> GPHMASMLEAKFEEASLFKRIIDGFKDCVQLVNFQCKEDGIIAQAVDDSRVLLVSLEIGVEAFQEYRCDHPVTLGMDLTSLSKILRCGNNTDTLTLIADNTPDSIILLFEDTKKDRIAEYSLKLMDIDADFLKIEELQYDSTLSLPSSEFSKIVRDLSQLSDSINIMITKETIKFVADGDIGSGSVIIKPFVDMEHPETSIKLEMDQPVDLTFGAKYLLDIIKGSSLSDRVGIRLSSEAPALFQFDLKSGFLQFFLAPKFNDEGSNSQSNGSGALEAKFEEASLFKRIIDGFKDCVQLVNFQCKEDGIIAQAVDDSRVLLVSLEIGVEAFQEYRCDHPVTLGMDLTSLSKILRCGNNTDTLTLIADNTPDSIILLFEDTKKDRIAEYSLKLMDIDADFLKIEELQYDSTLSLPSSEFSKIVRDLSQLSDSINIMITKETIKFVADGDIGSGSVIIKPFVDMEHPETSIKLEMDQPVDLTFGAKYLLDIIKGSSLSDRVGIRLSSEAPALFQFDLKSGFLQFFLAPKFNDEGSNSQASNSGALEAKFEEASLFKRIIDGFKDCVQLVNFQCKEDGIIAQAVDDSRVLLVSLEIGVEAFQEYRCDHPVTLGMDLTSLSKILRCGNNTDTLTLIADNTPDSIILLFEDTKKDRIAEYSLKLMDIDADFLKIEELQYDSTLSLPSSEFSKIVRDLSQLSDSINIMITKETIKFVA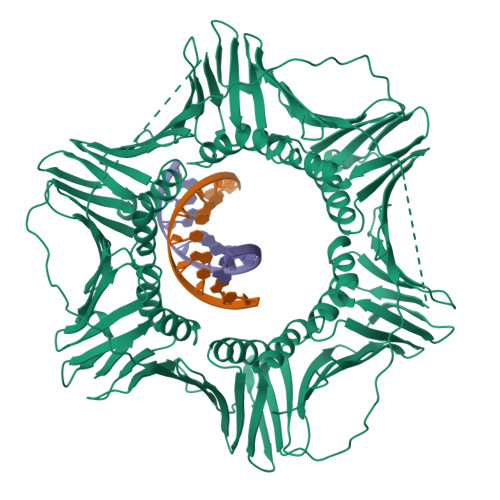DGDIGSGSVIIKPFVDMEHPETSIKLEMDQPVDLTFGAKYLLDIIKGSSLSDRVGIRLSSEAPALFQFDLKSGFLQFFLAPKFNDEE>SSQIRQNYSTDVEAAVNSLVNLYLQASYTYLSLGFYFDRDDVALEGVSHFFRELAEEKREGYERLLKMQNQRGGRALFQDIKKPAEDEWGKTPDAMKAAMALEKKLNQALLDLHALGSARTDPHLCDFLETHFLDEEVKLIKKMG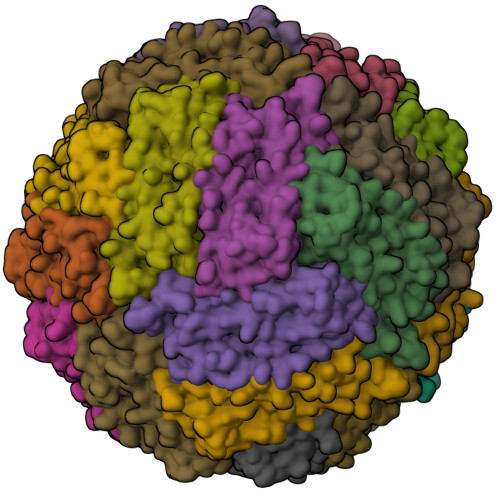DHLTNLHRLGGPEAGLGEYLFERLTLK[24x]2-[O-PHOSPHONOPYRIDOXYL]-AMINO-PENTANOIC ACID | C13 H21 N2 O7 P 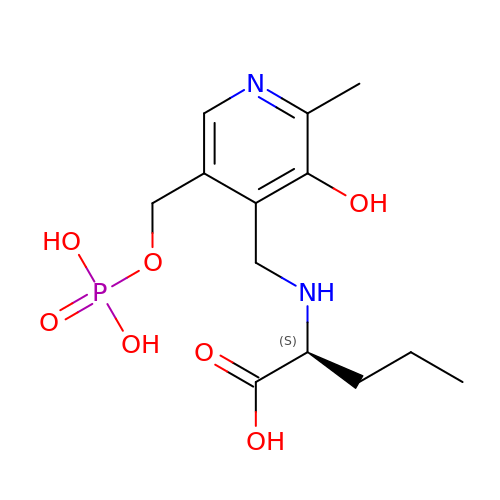| YYAMSLLSQINIQO-NSHDSACASA-N methyl 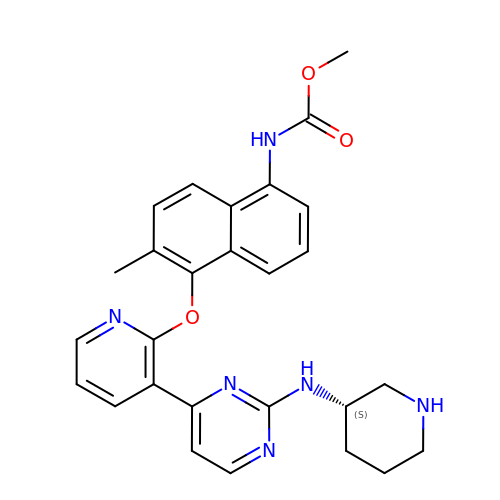~{N}-[6-methyl-5-[3-[2-[[(3~{S})-piperidin-3-yl]amino]pyrimidin-4-yl]pyridin-2-yl]oxy-naphthalen-1-yl]carbamate | C27 H28 N6 O3 | FMMZPTONJKUBJE-SFHVURJKSA-N> MAFRATLSFAGKEFDVLDCTYSL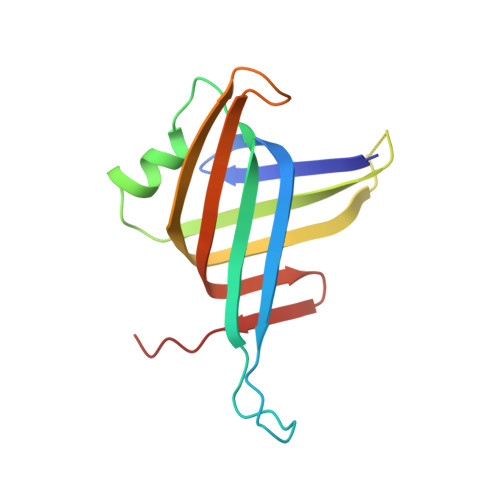KRDVDSKGRPSSNIYGGQIRLHVESTDDTSILENMTNQFKPHSGSIVFKKGDEEAKMKELTWENGYITEFTENIDIVGSQPMTITFVVSAQVIKIGGAQFEQNWPK> MIVNVIQKDRLKEQKLQFIRNHQQAFD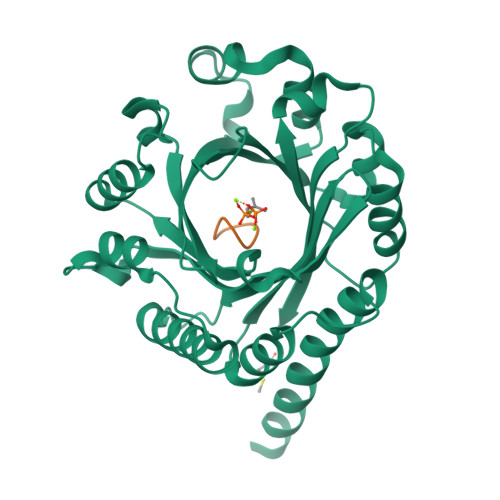VEPIYPLPLFEDFVTSIEGDCSLEASCKIESDKLIASRFLLFFEDKTQEWQKYLHQSLTFFGLVENRVGVKINYSLLQQFLGSSFDFSKVTVLSAGIDLRNNLAESSLKMHIRIKDYPEKLDKAFALSDGAADGNYLKDFVNLIGFDFYFNGKSEIEIYAEVQEDDFFKPEINNLVWQHFPKTALQPLKASSLFFTGLSKANNNPVLYYHLKNRQDLTNYFKLNDTAQRVHSFYQHQDILPYMWVGTAQKELEKTRIENIRLYYYKSFKMESN;> INPYLYP> F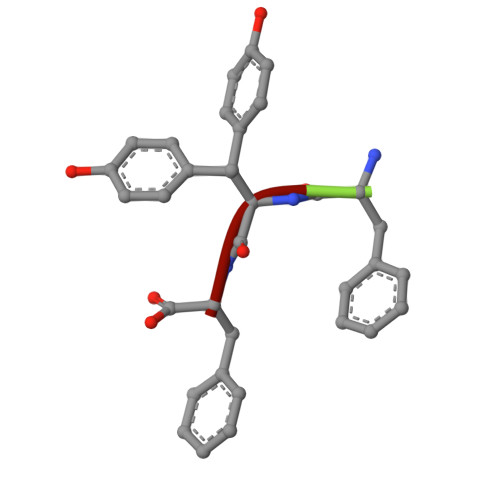YF>[4x]MDYKDDDDKEPGGARLRLQRTGGLGGERERQPCGDGNTETHRAPDLVQWTRHMEAVKAQLLEQAQGQLRELLDRAMREAIQSYPSQDKPLPPPPPGSLSRTQEPSLGKQKVFIIRKSLLDELMEVQHFRTIYHMFIAGLCVFIISTLAIDFIDEGRLLLEFDLLIFSFGQLPLALVTWVPMFLSTLLAPYQALRLWARGTWTQATGLGCALLAAHAVVLCALPVHVAVEHQLPPASRCVLVFEQVRFLMKSYSFLREAVPGILRARRGEGIQAPSFSSYLYFLFCPTLIYRETYPRT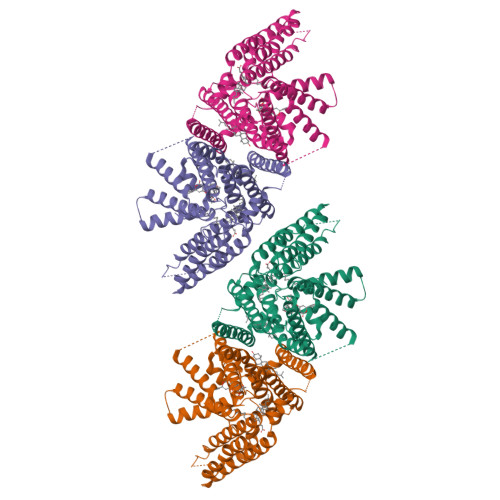PYVRWNYVAKNFAQALGCVLYACFILGRLCVPVFANMSREPFSTRALVLSILHATLPGIFMLLLIFFAFLHCWLNAFAEMLRFGDRMFYRDWWNSTSFSNYYRTWNVVVHDWLYSYVYQDGLRLLGARARGVAMLGVFLVSAVAHEYIFCFVLGFFYPVMLILFLVIGGMLNFMMHDQRTGPAWNVLMWTMLFLGQGIQVSLYCQEWYARRHCPLPQATFWGLVTPRSWSCHT> MLRCSCACRRGVYHNAPSVYPFVKPFHDTPYDQDRGRHDSVGQRYRKNSWPEWM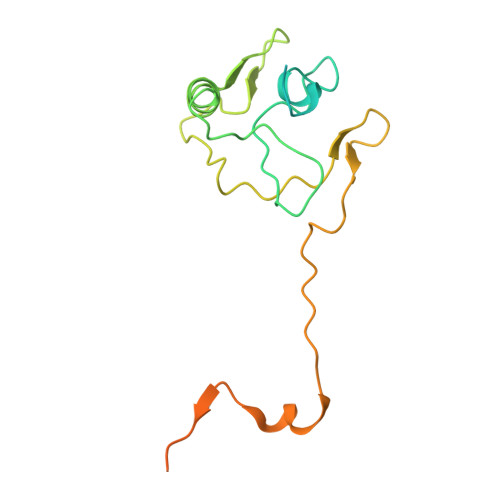DNGADGTGYGIGLHRTHPLSRLRGNLKRSPSHVPRVLGMMIQGVWHKSGVKLYFRGGKPPNPSVHPYLTGEPCPLYGWKVTDESVIRQFNMPSIDGTNFRYKPYVALQERKIMGVQVPSDSVSLASGRTTESKPLAKRLFFWR> MERFLLNSTVLLYRLSTVSLDEVSLDERVESSVFLAQYEQARSLPDHVAKSAWSYLVQQIKQRNMKLGPVAILRLIAEKFIKNEKGGPKIDLPMFSEWQTLMSRVSCLPIIACHQVFNPGPASQEYSFRWPLYPYHPTVEDYITRECLHETHQHLNGSTSAEECWLDALKHPEACLRDFEKGWASQEMKQLCAQIDPSLTPRIFKDRLQIACNIREILCRVAQGVELPEWIASMQNPQQLANSTILHNGREYGFATVWPIDDKYSQESEFCWLTGLLEKWRFNAPEGLERLLWIYLLIQNQYLTLLVQRDDFFGFEQFQNYTMTELREETEKSYLSRFKHAHGAGVYSQVRYLEGRFAPKSDPNKMQKLLFSVLRGYWEYLSAHMSMEWVHEKPLTISQVLDNLELVEPHGKCVELALVPHFIKRKPKNGEAYPHALLFKDLKNQAAILMDMLKSEPRLTGWIRGVDAAANEMHAPPELFCPLFRVLAKSGIAHFTYHVGEDFPHLISGIRSIDDAL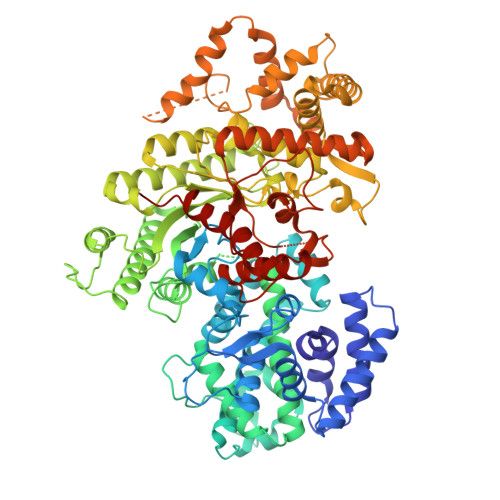RFLPLRNGDRLGHCTAIGITPSIWKRSLPLSLSMTKETRLLDLVFIWRELRSHPELLRYASDAAIEAVRLAHKVFSLEEEVSITTLDQVFEMRGLLAESEGLLSELNEPLKPKSLWLEEYERARELVKTTGMKRPLKLYKQWLTSDNVRKQRAEYVEVALEYLPDEAVVALQQAVMAKMADRNIAIECPPTSNTRISQYRNVSEHHIFRWMGLPGEAIEGDVPMSICLGSDDPGIFAADLKSEFYHLFVVLTRKFGLSPADALRKVAEVNENGRIYRFHDVS>[3x]MKHHHHHHSGAMMSGPTTDTPAAIQICRIMRPDDANVAGNVHGGTILKMIEEAGAIIST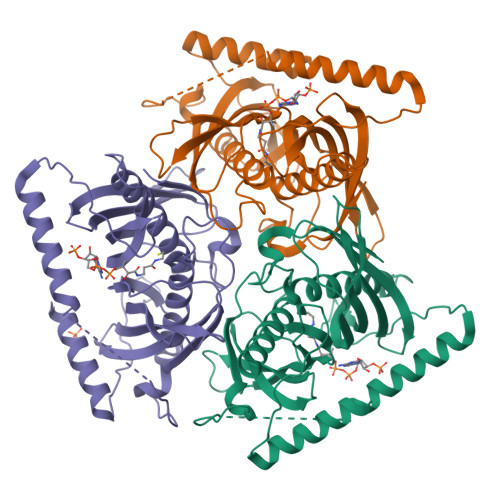RHCNSQNGERCVAALARVERTDFLSPMCIGEVAHVSAEITYTSKHSVEVQVHVMSENILTGTKKLTNKATLWYVPLSLKNVDKVLEVPPIVYLRQEQEEEGRKRYEAQKLERMETKWRNGDIVQPVLNPEPNTVSYSQSSLIHLVGPSDCTLHGFVHGGVTMKLMDEVAGIVAARHCKTNIVTASVDAINFHDKIRKGCVITISGRMTFTSNKSMEIEVLVDADPVVDNSQKRYRAASAFFTYVSLNQEGKPMPVPQLVPETEDEKKRFEEGKGRYLQM> APTSSSTKKTQLQLEHLLLDLQMILNGINNYKNPKLTRMLTFKFYMPKKATELKHLQCLEEELKKLEEVLNLAQSKNFHLRPRDLISNINVIVLELKGSETTFMCEYADETATIVEFLNRWITFSQSIIS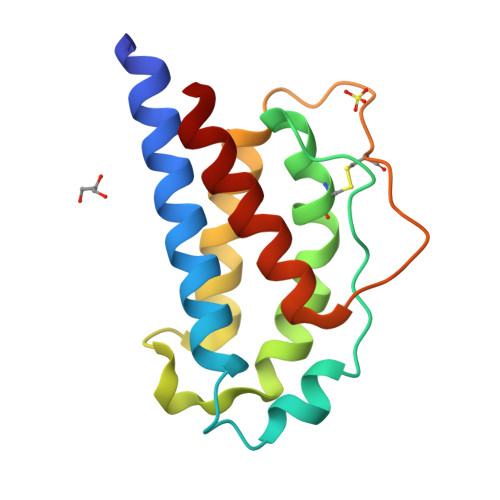TLT5-(2,5-DIMETHYL-3-THIENYL)-1H-PYRAZOLE-3-CARBOXAMIDE | C10 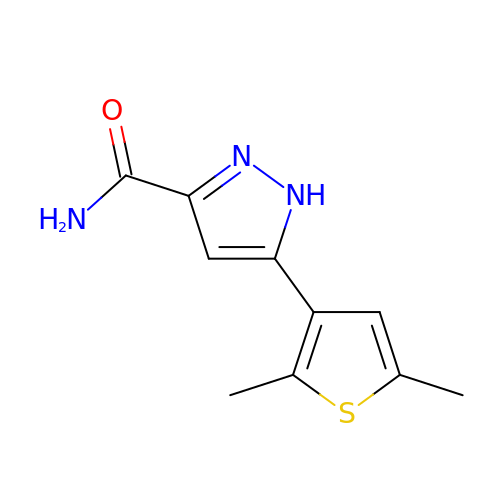H11 N3 O S | KLVHCUPVBQYXJT-UHFFFAOYSA-N>MSHPPSNTPPVKPGGLPLLGHILEFGKNPHAFLMALRHEFGDVAEFRMFHQRMVLLTGSQASEAFYRAPDEVLDQGPAYRIMTPIFGRGVVFDARIERKNQQLQMLMPALRDKPMRTYSEIIVAEVEAMLRDWKDAGTIDLLELTKELTIYTSSHCLLGAEFRHELNTEFAGIYRDLEMGIQPIAYVFPNLPLPVFKRRDQARVRLQELVTQIMERRARSQERSTNVFQMLIDASYDDGSKLTPHEITGMLIATIFAGHHTSSGTTAWVLIELLRRPEYLRRVRAEIDALFETHGRVTFESLRQMPQLENVIKEV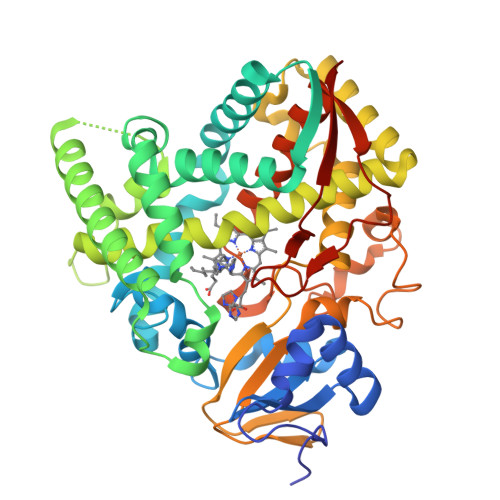LRLHPPLILLMRKVMKDFEVQGMRIEAGKFVCAAPSVTHRIPELFPNPELFDPDRYTPERAEDKDLYGWQAFGGGRHKCSGNAFAMFQIKAIVCVLLRNYEFELAAAPESYRDDYRKMVVEPASPCLIRYRRRDA[3x]> AECSVDIQGNDQMQFNTNAITVDKSCKQFTVNLSHPGNLPKNVMGHNWVLSTAADM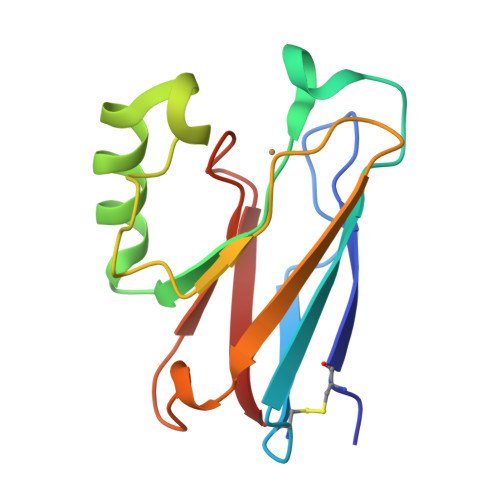QGVVTDGMASGLDKDYLKPDDSRVIAHTKLIGSGEKDSVTFDVSKLKEGEQYMFFCAAHAAMKGTLTLK>GPMSQPSYGPLFEALAHYNDKLLAMAKAQTERTAQALLQTNLDDLGQVLEQGSQQPWQLIQAQMNWWQDQLKLMQHTLLKSAGQPSEPVITPERSDRRFKAEAWSEQPIYDYLKQSYLLTARHLLASVDALEGVPQKSRERLRFFTRQYVNAMAPSNFLATNPELLKLTLESDGQNLVRGLALLAEDLERSADQLNIRLTDESAFELGRDLALTPGRVVQRTELYELIQYSPTTETVGKTPVLIVPPFINKYYIMDMRPQNSLVAWLVAQGQTVFMISWRNPGVAQAQIDLDDYVVDGVIAALDGVEAATGEREVHGIGYCIGGTALSLAMGWLAA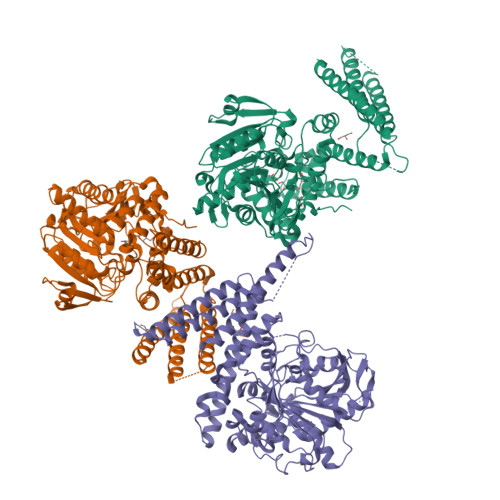RRQKQRVRTATLFTTLLDFSQPGELGIFIHEPIIAALEAQNEAKGIMDGRQLAVSFSLLRENSLYWNYYIDSYLKGQSPVAFDLLHWNSDSTNVAGKTHNSLLRRLYLENQLVKGELKIRNTRIDLGKVKTPVLLVSAVDDHIALWQGTWQGMKLFGGEQRFLLAESGHIAGIINPPAANKYGFWHNGAEAESPESWLAGATHQGGSWWPEMMGFIQNRDEGSEPVPARVPEEGLAPAPGHYVKVRLNPVFACPTEEDAA[3x]>SNAVTMGRIMRPDDANVAGNVHGGTILKMIEEAGAIISTRHCNSQNGERCVAALARVERTDFLSPMCIGEVAHVSAEITYTSKHSVEVQVHVMSENILTGTKKLTNKATLWYVPLSLKNVDKVLEVPPIVYLRQEQEEEGRKRYEAQKLERMETKWRNGDIVQPVLNPEPNTVSYSQSSLIHLVGPSDCTLHGFVHGGVTMKLMDEVAGIVAARHCKTNIVTASVD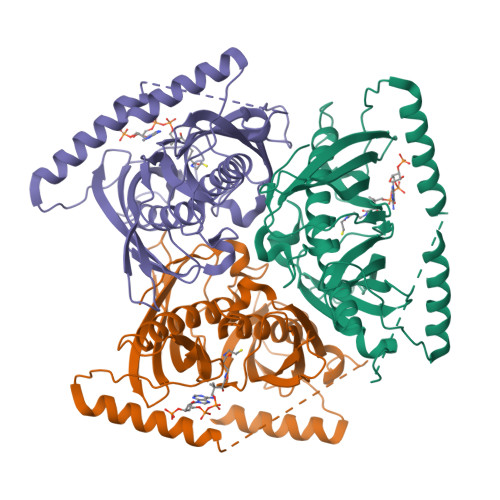AINFHDKIRKGCVITISGRMTFTSNKSMEIEVLVDADPVVDNSQKRYRAASAFFTYVSLNQEGKPMPVPQLVPETEDEKKRFEEGKGRYLQM[3x]>NQIVSGAAWTDTAGNTIQAHGAGILQVGSTFYWFGEDKSHNSALFKAVSCYTSSDLVNWSRQNDALSPIAGTMISTSNVVERPKVIFNQKNSEYVMWFHSDSSNYGAAMVGVATAKTPCGPYTYKGSFKPLGADSRDESIFQDDDSAQTAYLLYASDNNQNFKISRLDANYYNVTAQVSVMNGATLAAPGIVKHNGEYFLIASHTSGWAPNPNKWFSASSLAGPWSAQQDIAPSATRTWYSQNAFDLPLGSNAIYMGDRWRPSLLGSSRYIWYPLDFSSGAPQIVHADVWSVNVQAGTYSVASGTSYEAENGQRGGSSTILSGSGFSGGKAVGYLGHGGTVTINNVQSNGGSHWVALY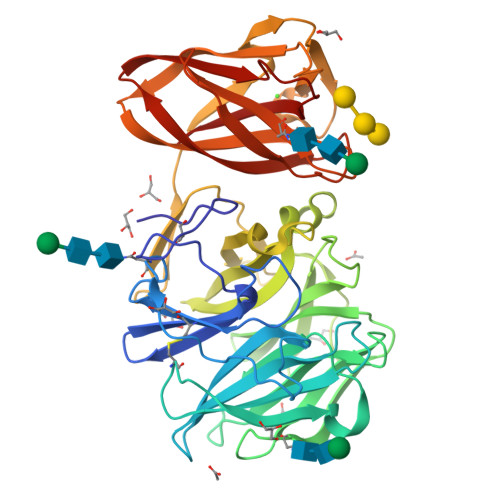FANGDSTYRNVTVSVNGGPSVLVDQPDSGGGNVVISVPVKLNLNSGENSITFGSGQSNYAADLDKIIVY[4x]> QKDLKLGELLLQKGWISREAL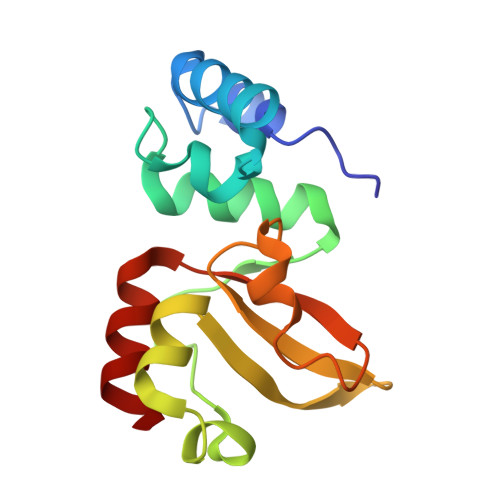EEALVEQEKTGDLLGRILVRKGLPEEALYRALAEQKGLEFLESTEGIVPDPSAALLLLRSDALRYGAVPIGFQNGEVEVVLSDPRHKEAVAQLLNRPARFYLALPQAWEELFRRAY> SDRVRSITLGNSTITTQESANVVVGYGVWPDYLSDEEATAEDQPTQPDVATCRFYTLDSVSWMKESQGWWWKFPDALRDMGLFGQNMQYHYLGRSGYTIHVQCNASKFHQGCLLVVCVPEAEMGAANINEKINREHLSNGEVANTFSGTKSSNTNDVQQAVFNAGMGVAVGNLTIFPHQWINLRTNNCATIV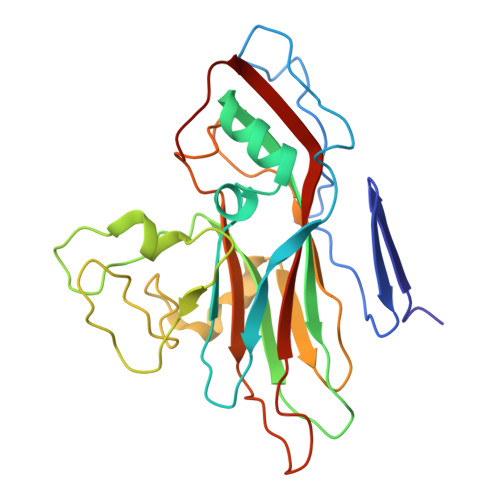MPYINSVPMDNMFRHYNFTLMIIPFAKLDYAAGSSTYIPITVTVAPMCAEYNGLRLAGHQ> MLQKKPYNGLHEKELNQINQQDGSPCVAISAPGC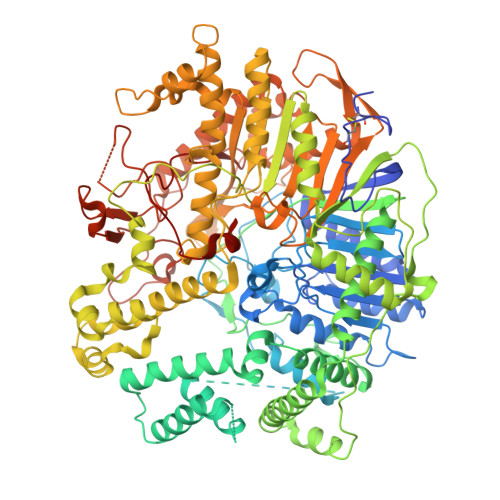FIKGSNLFSEKRAGNRVRFFTTGRDYFSDLASALDSASSSIFITGWQVNYDVLLDGRRSLWQCLRQALERSPALKVYVMPWLSPSGSLGTYDFETMLAVFQLNAGLEGGARAFCTPAIQQSDMQGLGVAFSHHQKSVVIDNRIGYVGGIDLAYGRRDDNDFSLDASGRRGNDAYNPGLPHLGWMAEDEHVSSMGLMMATLFDLSRPLASLTLHAPTLRLSPFPHIAASDEPLLSIPLAPSRARALNGAAYLSDLFRSPMLPSLQWLGRAYNSSKEGLDEGFERLDALRRQMVASSIRAIANLIADNLDALPIEPELERRLRAWLEELRTAALNLPEALRIKSLLLINQWMSETELGQVLTLISGKGFEDIPQNLSGKAGELAGSLFWTLHRLMQARAGGHQQPYRYLDEAPQPLASPDNARLAADQPRMPWQDVHCRIEGPSVYDLARNFIDRWNGQQAYLAKTPALQDTALVRSALEAVMKWLNSLAAAAGLENYLDEKRNLRLELDPPTPCWINAPEQLPQEPEVRRGGMTVQVLRSAAARMLEQEQAGRLGAGVNLPLQVGVSTEGVQSNCKDAMLLAISGAQQFIYIENQFFQSEFGKEGEVFKDLPLSGPMASLRDVGSLRRDFVVRIRLEEALEQRDLWLLDWAEVEKIAQEPGTEARQFLKSMLAMWGVNAQGWLTHKLGEAQHGLLNEIGEALARRIERAIQREHPFHVYLVLPVHPEGALNVPNIMHQVHLTQQSLVFGEQSLVKRIQRQMALKALEGKSDPAQAREIIERKDARGRPVYEQQDWSRYLTLLNLRTWAVLGGRVVTEQIYVHSKLLIADDRVAILGSANINDRSLQGERDSELAVMVRDSEPLTVRLDGKNDAIVGKAIHQLRVNLWKKHFGLSQGPGGFVKPASELSAYLSIPAAQEAWEAIQTLAKENTRAYERTFNFIPQNISQTQLQLTPEPPKGFEDGFPASIWPTWAYRKPGELRAGGQLMEPMPYQEIFWRSSNLTSVKTFPPPNGVSGFITALPTSWTRGERNDSGLNLSILAHQDSRSLPTQVAMNGDSSAQGKHRT Here we examined the factors that define the oligomeric state in a circular protein oligomer by studying the Bacillus trp RNA-binding attenuation protein (TRAP). Studies on B. subtilis have shown that when TRAP is activated by bound tryptophan, it can recognize and bind specific segments of RNA. When the tryptophan concentration is high transcription attenuation occurs as TRAP, binding to the leader RNA region of the trpEDCFBA operon transcript, induces the formation of a transcription terminator hairpin thus preventing the establishment of an antiterminator structure. When the concentration of tryptophan is limiting, TRAP is inactive, which allows transcription to proceed into the structural genes.

Previously determined X-ray structures of B. subtilis and B. stearothermophilus TRAP revealed 11-subunit oligomers with essentially identical architecture. We hypothesized that the 11-mer to 12-mer switch could be induced by withdrawal of the C-terminal amino acids from the subunit-subunit interface, as observed in B. halodurans TRAP. Such a switch could be engineered by simply removing the C-terminal amino acids starting from position 72. The conformation of individual subunits is also very similar, with the main chain r.m.s. difference with the B. halodrurans TRAP (residues 8–65) of 0.38 Å and 0.33 Å, respectively, for the engineered B. stearothermophilus and B. subtilis TRAP. The engineered 12-mer TRAP share almost identical intersubunit hydrogen bonding patterns with those in wild type 11-mers, Tables S2 and S3.

>SDFVVIKAVEDGVNVIGLTRGTDTKFHHSEKLDKGEVIIAQFTEHTSAIKVRGEALIQTAYGEMK[6x]> GKAE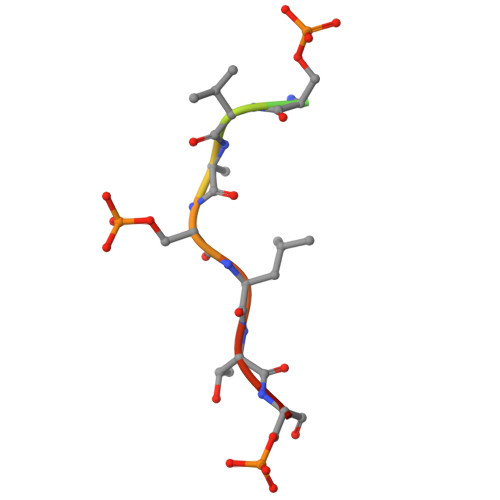SVASLTSQ(3R)-3-[(1S)-4-(acetylamino)-1-(3-chlorophenyl)-1-hydroxybutyl]-N-{(1S)-2-cyclohexyl-1-[(methylamino)methyl]ethyl}piperidine-1-carboxamide | C28 H45 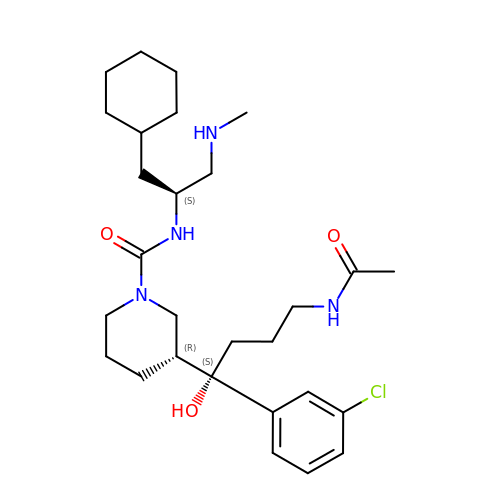Cl N4 O3 | PPGUIDOUTGLYCO-MAARLIENSA-N(7E)-6-methyl-8-[(4S)-2,6,6-trimethyl-4-oxidanyl-cyclohexen-1-yl]octa-3,5,7-trien-2-one | C18 H26 O2 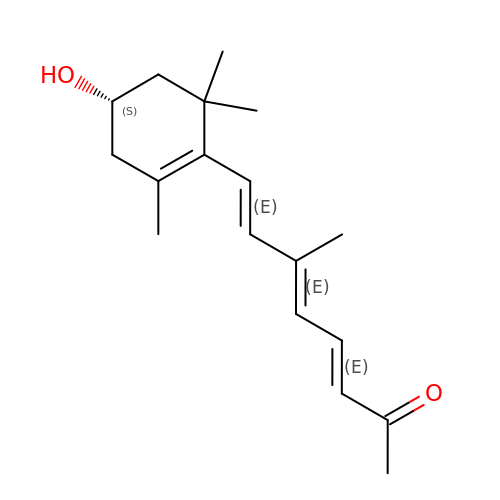| JLNMEHQAHDSEEE-FRIDJMAZSA-N> GSVHKHTGRNCGRKFKIGEPLYRCHECGCDDTCVLCIHCF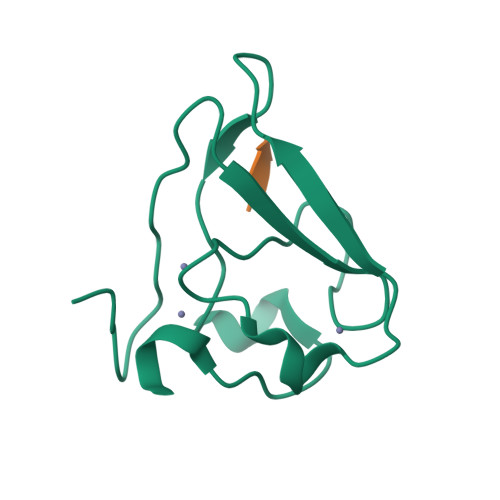NPKDHVNHHVCTDICTEFTSGICDCGDEEAWNSPLHCKAEEQ;> RIAAA>[2x]MAAPVVAPPGVVVSRANKRSGAGPGGSGGGGARGAEEEPPPPLQAVLVADSFDRRFFPISKDQPRVLLPLANVALIDYTLEFLTATGVQETFVFCCWKAAQIKEHLLKSKWCRPTSLNVVRIITSELYRSLGDVLRDVDAKALVRSDFLLVYGDVISNINITRALEEHRLRRKLEKNVSVMTMIFKESSPSHPTRCHEDNVVVAVDSTTNRVLHFQKTQGLRRFAFPLSLFQGSSDGVEVRYDLLDCHISICSPQVAQLFTDNFDYQTRDDFVRGLLVNEEILGNQIHMHVTAKEYGARVSNLHMYSAVCADVIRRWVYPLTPEANFTDSTTQSCTHSRHNIYRGPEVSLGHGSILEENVLLGSGTVIGSNCFITNSVIGPGCHIGDNVVLDQTYLWQGVRVAAGAQIHQSLLCDNAEVKERVTLKPRSVLTSQVVVGPNITLPEGSVISLHPPDAEEDEDDGEFSDDSGADQEKDKVKMKGYNPAEVGAAGKGYLWKAAGMNMEEEEELQQNLWGLKINMEEESESESEQSMDSEEPDSRGGSPQMDDIKVFQNEVLGTLQRGKEENISCDNLVLEINSLKYAYNISLKEVMQVLSHVVLEFPLQQMDSPLDSSRYCALLLPLLKAWSPVFRNYIKRAADHLEALAAIEDFFLEHEALGISMAKVLMAFYQLEILAEETILSWFSQRDTTDKGQQLRKNQQLQRFIQWLKEAEEESSEDD;>[2x]MPGSAAKGSELSERIESFVETLKRGGGPRSSEEMARETLGLLRQIITDHRWSNAGELMELIRREGRRMTAAQPSETTVGNMVRRVLKIIREEYGRLHGRSDESDQQESLHKLLTSGGLNEDFSFHYAQLQSNIIEAINELLVELEGTMENIAAQALEHIDSNEVIMTIGFSRTVEAFLKEAARKRKFHVIVAECAPFCQGHEMAVNLSKAGIETTVMTDAAIFAVMSRVNKVIIGTKTILANGALRAVTGTHTLALAAKHHSTPLIVCAPMFKLSPQFPNEEDSFHKFVAPEEVLPFTEGDILEKVSVHCPVFDYVPPELITLFISNIGGNAPSYIYRLMSELYHPDDHVL;>[2x]MAAVAVAVREDSGSGMKAELPPGPGAVGREMTKEEKLQLRKEKKQQKKKRKEEKGAEPETGSAVSAAQCQVGPTRELPESGIQLGTPREKVPAGRSKAELRAERRAKQEAERALKQARKGEQGGPPPKASPSTAGETPSGVKRLPEYPQVDDLLLRRLVKKPERQQVPTRKDYGSKVSLFSHLPQYSRQNSLTQFMSIPSSVIHPAMVRLGLQYSQGLVSGSNARCIALLRALQQVIQDYTTPPNEELSRDLVNKLKPYMSFLTQCRPLSASMHNAIKFLNKEITSVGSSKREEEAKSELRAAIDRYVQEKIVLAAQAISRFAYQKISNGDVILVYGCSSLVSRILQEAWTEGRRFRVVVVDSRPWLEGRHTLRSLVHAGVPASYLLIPAASY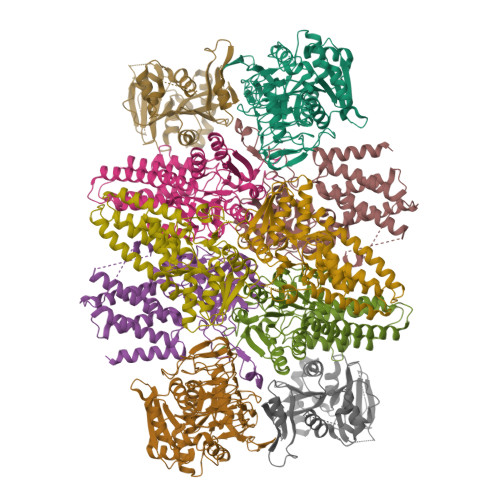VLPEVSKVLLGAHALLANGSVMSRVGTAQLALVARAHNVPVLVCCETYKFCERVQTDAFVSNELDDPDDLQCKRGEHVALANWQNHASLRLLNLVYDVTPPELVDLVITELGMIPCSSVPVVLRVKSSDQ;>MDDKELIEYFKSQMKEDPDMASAVAAIRTLLEFLKRDKGETIQGLRANLTSAIETLCGVDSSVAVSSGGELFLRFISLASLEYSDYSKCKKIMIERGELFLRRISLSRNKIADLCHTFIKDGATILTHAYSRVVLRVLEAAVAAKKRFSVYVTESQPDLSGKKMAKALCHLNVPVTVVLDAAVGYIMEKADLVIVGAEGVVENGGIINKIGTNQMAVCAKAQNKPFYVVAESFKFVRLFPLNQQDVPDKFKYKADTLKVAQTGQDLKEEHPWVDYTAPSLITLLFTDLGVLTPSAVSDELIKLYL[2x];>MEFQAVVMAVGGGSRMTDLTSSIPKPLLPVGNKPLIWYPLNLLERVGFEEVIVVTTRDVQKALCAEFKMKMKPDIVCIPDDADMGTADSLRYIYPKLKTDVLVLSCDLITDVALHEVVDLFRAYDASLAMLMRKGQDSIEPVPGQKGKKKAVEQRDFIGVDSTGKRLLFMANEADLDEELVIKGSILQKHPRIRFHTGLVDAHLYCLKKYIVDFLMENGSITSIRSELIPYLVRKQFSSASSQQGQEEKEEDLKKKELKSLDIYSFIKEANTLNLAPYDACWNACRGDRWEDLSRSQVRCYVHIMKEGLCSRVSTLGLYMEANRQVPKLLSALCPEEPPVHSSAQIVSKHLVGVDSLIGPETQIGEKSSIKRSVIGSSCLIKDRVTITNCLLMNSVTVEEGSNIQGSVICNNAVIEKGADIKDCLIGSGQRIEAKAKRVNEVIVGNDQLMEI[2x]>GTTTTGXCAA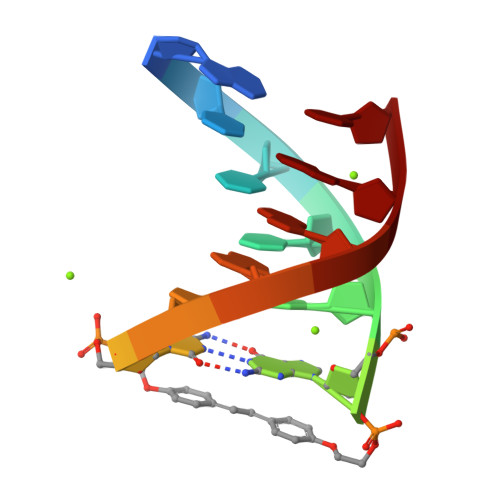AAC[2x]(4-hydroxyphenyl)acetonitrile | C8 H7 N O | 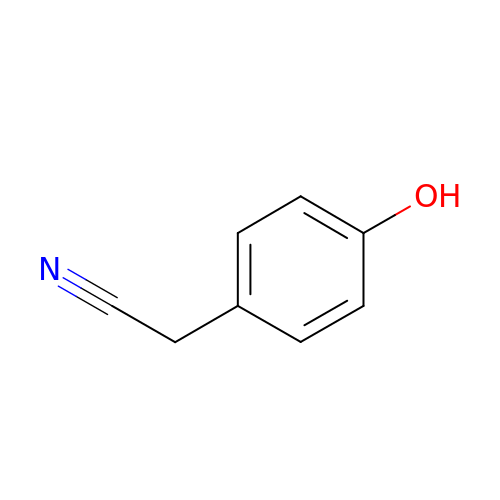AYKYOOPFBCOXSL-UHFFFAOYSA-N> ADSGEGDFLAEGGGVRGPRVVERHQSACKDSDWPFCSDEDWNYKCPSGCRMKGLIDEVNQDFTNRINKLKNSLFEYQKNNKDSHSLTTNIMEILRGDFSSANNRDNTYNRVSEDLRSRIEVLKRKVIEK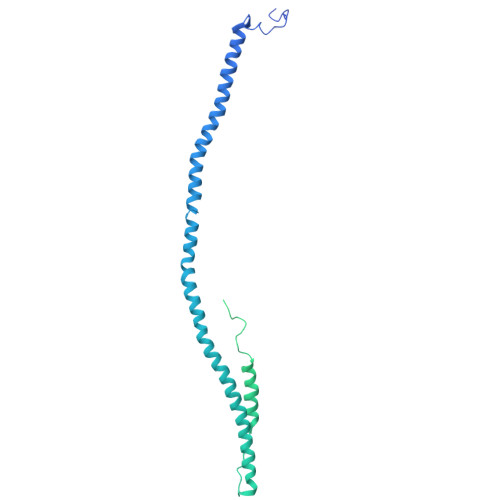VQHIQLLQKNVRAQLVDMKRLEVDIDIKIRSCRGSCSRALAREVDLKDYEDQQKQLEQVIAKDLLPSRDRQHLPLIKMKPVPDLVPGNFKSQLQKVPPEWKALTDMPQMRMELERPGGNEITRGGSTSYGTGSETESPRNPSSAGSWNSGSSGPGSTGNRNPGSSGTGGTATWKPGSSGPGSTGSWNSGSSGTGSTGNQNPGSPRPGSTGTWNPGSSERGSAGHWTSESSVSGSTGQWHSESGSFRPDSPGSGNARPNNPDWGTFEEVSGNVSPGTRREYHTEKLVTSKGDKELRTGKEKVTSGSTTTTRRSCSKTVTKTVIGPDGHKEVTKEVVTSEDGSDCPEAMDLGTLSGIGTLDGFRHRHPDEAAFFDTASTGKTFPGFFSPMLGEFVSETESRGSESGIFTNTKESSSHHPGIAEFPSRGKSSSYSK> SKVVYVSHDGTRRELDVADGVSLMQAAVSNGIYDIVGDCGGSASCATCHVYVNEAFTDKVPAANEREIGMLESVTAELKPNSRLSCQIIM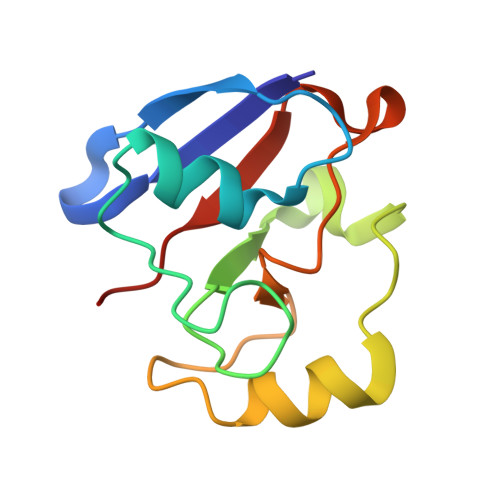TPELDGIVVDVPDRQW> GAMAKVQVNNVVVLDNPSPFYNPFQFEITFECIEDLSEDLEWKIIYVGSAESEEYDQVLDSVLVGPVPAGRHMFVFQADAPNPGLIPDADAVGVTVVLITCTYRGQEFIRVGYYV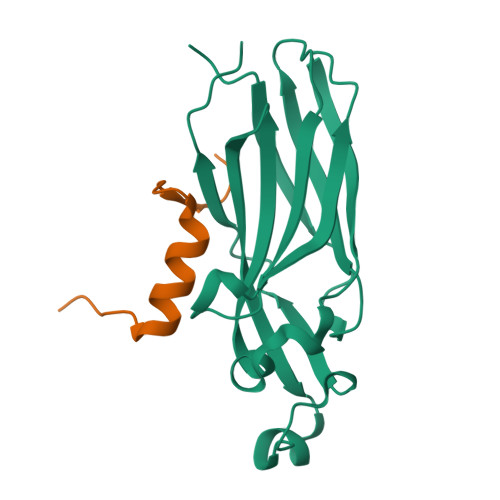NNEYTETELRENPPVKPDFSKLQRNILASNPRVTRFHINWEDN;> GAMGTLTPKEAELARRIRGAGGRTLNGFG2-({2-chloro-6-[(2,4-dichlorophenyl)sulfanyl]benzyl}carbamoyl)benzoic 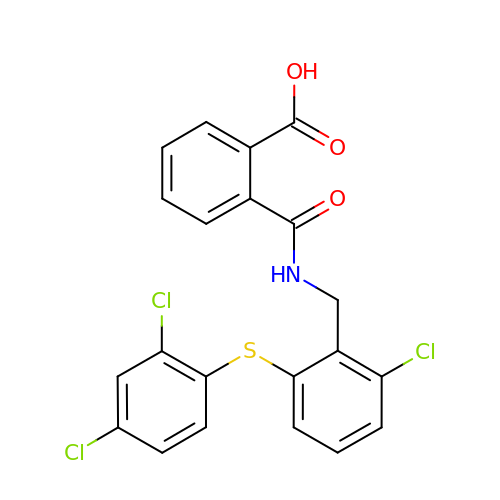acid | C21 H14 Cl3 N O3 S | HLWGMGIORMMWMJ-UHFFFAOYSA-N>[2x]MAHHHHHHSAALEVLFQ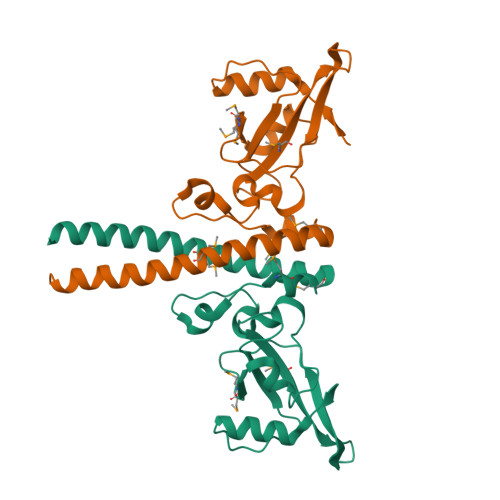GPGMASGSNVEEYELDVEALVVILRDRNIPRNPLHGEVIGLRLTEGWWGQIERFQMVRLILQNDDNEPLQRPRYEVIQRAVNPHTMFMISGPLAELQLAFQDLDLPEGPLRFGPLANGHYVQGDPYSSSYRPVTMAETAQMTRDELEDVLNTQSEIEIQMINLLELYEVETRALRRQLAERS> MNLFTPRSEINPTTTQELLYAYTGPAPVAYGTRTRAVLENIIRPYQYFYKEPNVQRALDIKTGCKEPEDINVEGPSSGFHTASVLKLADNFFRKYRPAMEKLKYWILVKLPKLKYAELSKGRQTYSFIHKRNLPAPIALEETVEFLEQNLRRKIGPTLLSYCQAIADVMELDETTYEGARDPRPWDIQLEEIDSDEEDPLFRQVGREETYTIKFSREELWDQMRTLNTMWKHLERGRLNRRTIATPSMLIRGFVKIVEDAAKEILENVPTSGVPVGGEEKLAKLASKQTFHTAVTGELSGDQEKFNECLDPDAMRLMWTVFLRKLGCPDWIMELFNIPFMVFKSKLADMGEGLVYTKGKLTDRKPLGEMPSEFDDLVRNVVGNSISCRLGMFMGMYNLTSTLLALISIEREELTGSHVESSDDFIHFFNCKTHEEMFKQAETLRLTLKLVGINMSPSKCILISPAGIGEFNSKFHHRDFVGNVATELPALVPNGTNPMTDLAMGLNVIKHSVNTGQMNLCTGALAMRIFNHAYKYAYMALGVTRRTRFMEENAITPLLTNQGASPVHSFSTMHLDEVALRRHLGLLDEETLRRILNPNNPVTQKGDPSMFFRIENKMPQIMEDYSVPSCFKYTLSRNRTIQDKPHKALLNKEERYQRVTSIINKLFPEVLIQEASAPGTVRESLKRRLELVV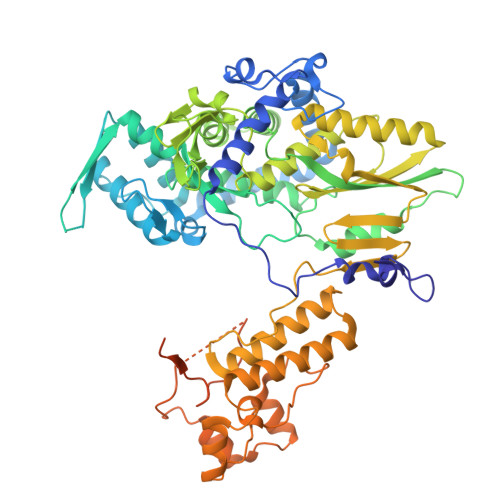ERSDLDEERKKRILSRIF>[2x]MASMTGGQQMGRDEAGITGTWYNQLGSTFIVTAGADGALTGTYESAAGKAESRYVLTGRYDSAPATDGSGTALGWTVAWKNNYRNAHSATTWSGQYVGGAEARINTQWLLTMGATEANGWASTLVGHDTFTKVKPSAASIDAAKKAGVNNGNPLDAVQQ

We describe here the use of an artificial cofactor employing the well‐known biotin‐streptavidin system to catalyze a Baylis‐Hillman reaction. As protein host, we chose streptavidin, as it can be easily crystallized and thereby supports the design process. There are several examples using streptavidin as the host for these cofactors, since its natural ligand biotin binds strongly (K d∼10−15 M) and is easy to modify with catalysts at the carboxylic acid group. No enzyme is known to naturally catalyze the Baylis‐Hillman reaction, a very versatile and atom‐economic C−C bond forming reaction for the production of various functionalized compounds and intermediates of active pharmaceutical ingredients (APIs).

We chose a derivative of DMAP as the artificial cofactor due to its low steric demand, which will facilitate its inclusion into the protein scaffold. The protein host around the cofactor was rationally designed on the basis of high‐resolution crystal structures obtained after each variation of the amino acid sequence. The location of the catalyst is in a shallow cavity at the surface of the protein. The system was evolved through repeated cycles of mutagenesis, activity tests, and structure determination. According to the presented structures and calculations the catalytically active site is too shallow to undergo interactions with 1.> MIEIKDKQLTGLRFIDLFAGLGGFRLALESCGAECVYSNEWDKYAQEVYEMNFGEKPEGDITQVNEKTIPDHDILCAGFPCQAFSISGKQKGFEDSRGTLFFDIARIVREKKPKVVFMENVKNFASHDNGNTLEVVKNTMNELDYSFHAKVLNALDYGIPQKRERIYMICFRNDLNIQNFQF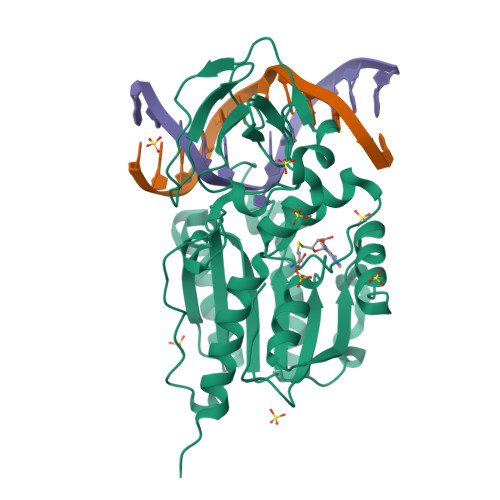PKPFELNTFVKDLLLPDSEVEHLVIDRKDLVMTNQEIEQTTPKTVRLGIVGKGGQGERIYSTRGIAITLSAYGGGIFAKTGGYLVNGKTRKLHPRECARVMGYPDSYKVHPSTSQAYKQFGNSVVINVLQYIAYNIGSSLNFKPY> GMSGDILNDIVAACLE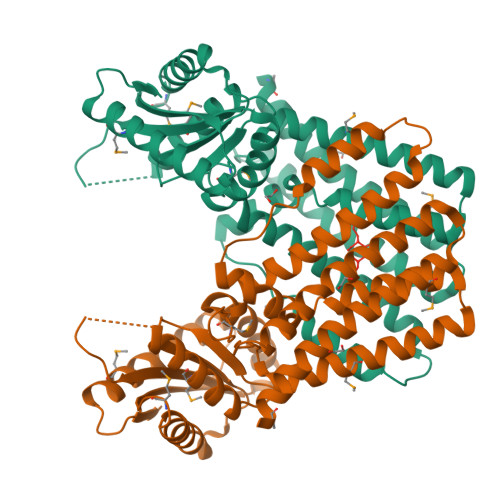LERKASSVFKMFAAHAGSDEARRFWETVADETRHHSAVYERLQERGGRENLPIIIYKPAETLEELEMIGKSIDEQVERYTEAPSSEAACLLGFRLQLYLLHPAFASLCRLTRDASGEDLPDIGYGRYLRRFIDGIGSCGLATAETELLGEALFRLWNEARQLAAQSHFDALTGVMTRAGFFKTVGSLAYAAQRSGSNVGIMLIDLDYFKLVGDNYGHQTGDRILQLVAETITSHLRRSDVVGRYDGDEFVVYLSPVEPASLRTVAENLRRSIEEESARMVPVTASIGVAQGILGTDVDGGIEELVRLADECLMQAKYTGKNKVVVK> GPKSWVEETCESIDTPECPAEFESPPTLLFSLDGFRAEYLHTWGGLLPVISKLKNCGTYTKNMRPMYPTKAFPNHYSIVTGLYPESHGIIDNKMYDPKMNA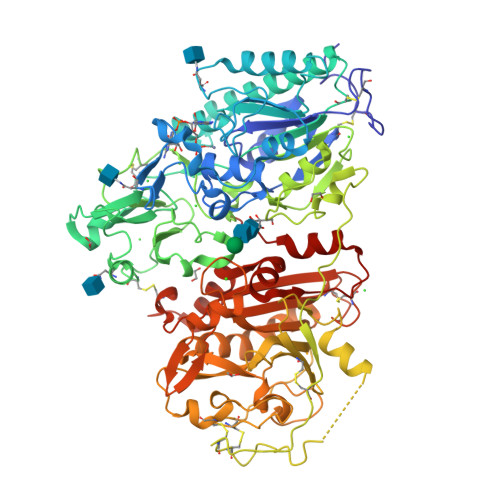SFSLKSKEKFNPLWYKGQPIWVTANHQEVKSGTYFWPGSDVEIDGILPDIYKVYNGSVPFEERILAVLEWLQLPSHERPHFYTLYLEEPDSSGHSHGPVSSEVIKALQKVDRLVGMLMDGLKDLGLDKCLNLILISDHGMEQGSCKKYVYLNKYLGDVNNVKVVYGPAARLRPTDVPETYYSFNYEALAKNLSCREPNQHFRPYLKPFLPKRLHFAKSDRIEPLTFYLDPQWQLALNPSERKYCGSGFHGSDNLFSNMQALFIGYGPAFKHGAEVDSFENIEVYNLMCDLLGLIPAPNNGSHGSLNHLLKKPIYNPSHPKEEGFLSQCPIKSTSNDLGCTCDPWIVPIKDFEKQLNLTTEDDDIYHMTVPYGRPRILLKQHRVCLLQQQQFLTGYSLDLLMPLWASYTFLSNDQFSRDDFSNCLYQDLRIPLSPVHKCSYYKSNSKLSYGFLTPPRLNRVSNHIYSEALLTSNIVPMYQSFQVIWHYLHDTLLQRYAHERNGINVVSGPVFDFDYDGRYDSLEILKQNSRVIRSQEILIPTHFFIVLTSCKQLSETPLECSALESSAYILPHRPDNIESCTHGKRESSWVEELLTLHRARVTDVELITGLSFYQDRQESVSELLRLKTHLPIFSQED> MQNSQDFSITELSLPKGGGAITGMGEALTPTGPDGMAALSLPLPISAGRGYAPAFTLNYNSGAGNSPFGLGWDCNVMTIRRRTHFGVPHYDETDTFLGPEGEVLVVADQPRDESTLQGINLGATFTVTGYRSRLESHFSRLEYWQPKTTGKTDFWLIYSPDGQVHLLGKSPQARISNPSQTTQTAQWLLEASVSSRGEQIYYQYRAEDDTGCEADEITHHLQATAQRYLHIVYYGNRTASETLPGLDGSAPSQADWLFYLVFDYGERSNNLKTPPAFSTTGSWLCRQDRFSRYEYGFEIRTRRLCRQVLMYHHLQALDSKITEHNGPTLVSRLILNYDESAIASTLVFVRRVGHEQDGNVVTLPPLELAYQDFSPRHHAHWQPMDVLANFNAIQRWQLVDLKGEGLPGLLYQDKGAWWYRSAQRLGEIGSDAVTWEKMQPLSVIPSLQSNASLVDINGDGQLDWVITGPGLRGYHSQRPDGSWTRFTPLNALPVEYTHPRAQLADLMGAGLSDLVLIGPKSVRLY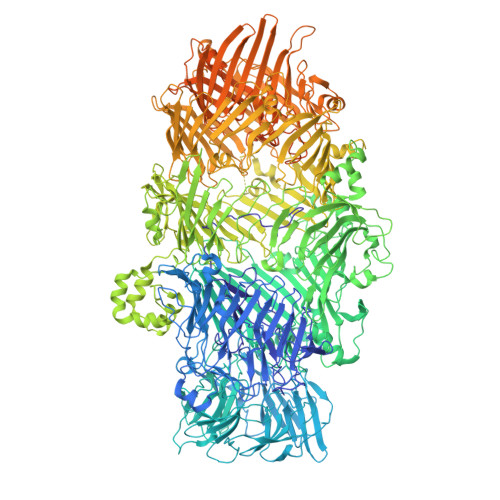ANTRDGFAKGKDVVQSGDITLPVPGADPRKLVAFSDVLGSGQAHLVEVSATKVTCWPNLGRGRFGQPITLPGFSQPATEFNPAQVYLADLDGSGPTDLIYVHTNRLDIFLNKSGNGFAEPVTLRFPEGLRFDHTCQLQMADVQGLGVASLILSVPHMSPHHWRCDLTNMKPWLLNEMNNNMGVHHTLRYRSSSQFWLDEKAAALTTGQTPVCYLPFPIHTLWQTETEDEISGNKLVTTLRYARGAWDGREREFRGFGYVEQTDSHQLAQGNAPERTPPALTKNWYATGLPVIDNALSTEYWRDDQAFAGFSPRFTTWQDNKDVPLTPEDDNSRYWFNRALKGQLLRSELYGLDDSTNKHVPYTVTEFRSQVRRLQHTDSRYPVLWSSVVESRNYHYERIASDPQCSQNITLSSDRFGQPLKQLSVQYPRRQQPAINLYPDTLPDKLLANSYDDQQRQLRLTYQQSSWHHLTNNTVRVLGLPDSTRSDIFTYGAENVPAGGLNLELLSDKNSLIADDKPREYLGQQKTAYTDGQNTTPLQTPTRQALIAFTETTVFNQSTLSAFNGSIPSDKLSTTLEQAGYQQTNYLFPRTGEDKVWVAHHGYTDYGTAAQFWRPQKQSNTQLTGKITLIWDANYCVVVQTRDAAGLTTSAKYDWRFLTPVQLTDINDNQHLITLDALGRPITLRFWGTENGKMTGYSSPEKASFSPPSDVNAAIELKKPLPVAQCQVYAPESWMPVLSQKTFNRLAEQDWQKLYNARIITEDGRICTLAYRRWVQSQKAIPQLISLLNNGPRLPPHSLTLTTDRYDHDPEQQIRQQVVFSDGFGRLLQAAARHEAGMARQRNEDGSLIINVQHTENRWAVTGRTEYDNKGQPIRTYQPYFLNDWRYVSNDSARQEKEAYADTHVYDPIGREIKVITAKGWFRRTLFTPWFTVNEDENDTAAEVKKVKMMKNIDPKLYQKTPTVSVYDNRGLIIRNIDFHRTTANGDPDTRITRHQYDIHGHLNQSIDPRLYEAKQTNNTIKPNFLWQYDLTGNPLCTESIDAGRTVTLNDIEGRPLLTVTATGVIQTRQYETSSLPGRLLSVAEQTPEEKTSRITERLIWAGNTEAEKDHNLAGQCVRHYDTAGVTRLESLSLTGTVLSQSSQLLIDTQEANWTGDNETVWQNMLADDIYTTLSTFDATGALLTQTDAKGNIQRLAYDVAGQLNGSWLTLKGQTEQVIIKSLTYSAAGQKLREEHGNDVITEYSYEPETQRLIGIKTRRPSDTKVLQDLRYEYDPVGNVISIRNDAEATRFWHNQKVMPENTYTYDSLYQLISATGREMANIGQQSHQFPSPALPSDNNTYTNYTRTYTYDRGGNLTKIQHSSPATQNNYTTNITVSNRSNRAVLSTLTEDPAQVDALFDAGGHQNTLISGQNLNWNTRGELQQVTLVKRDKGANDDREWYRYSGDGRRMLKINEQQASNNAQTQRVTYLPNLELRLTQNSTATTEDLQVITVGEAGRAQVRVLHWESGKPEDIDNNQLRYSYDNLIGSSQLELDSEGQIISEEEYYPYGGTALWAARNQTEASYKTIRYSGKERDATGLYYYGYRYYQPWIGRWLSSDPAGTIDGLNLYRMVRNNPVTLLDPDGLMPTIAERIAALKKNKVTDSAPSPANATNVAINIRPPVAPKPSLPKASTSSQPTTHPIGAANIKPTTSGSSIVAPLSPVGNKSTSEISLPESAQSSSSSTTSTNLQKKSFTLYRADNRSFEEMQSKFPEGFKAWTPLDTKMARQFASIFIGQKDTSNLPKETVKNISTWGAKPKLKDLSNYIKYTKDKSTVWVSTAINTEAGGQSSGAPLHKIDMDLYEFAIDGQKLNPLPEGRTKNMVPSLLLDTPQIETSSIIALNHGPVNDAEISFLTTIPLKNVKPHKR> GPEGERKNNNKRWYFTREQLENSPSRRFGVDPDKELSYRQQAANLLQDMGQRLNVSQLTINTAIVYMHRFYMIQSFTRFPGNSVAPAALFLAAKVEGQPKKLEHVIKVAHTCLHPQESLPDTRSEAYLQQVQDLVILESIILQTLGFELTIDHPHTHVVKCTQLVRASKDLAQTSYFMATNSL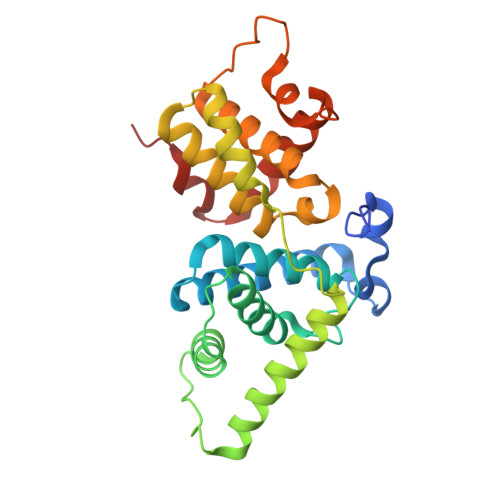HLTTFSLQYTPPVVACVCIHLACKWSNWEIPVSTDGKHWWEYVDATVTLELLDELTHELLQILEKTPNRLKRIWNWR> MALRGTVTDFSGFDGRADAEVLRKAMKGLGTDEDSILNLLTARSNAQRQQIAEEFKTLFGRDLVNDMKSELSGKFEKLIVALMKPSRLYDAYEL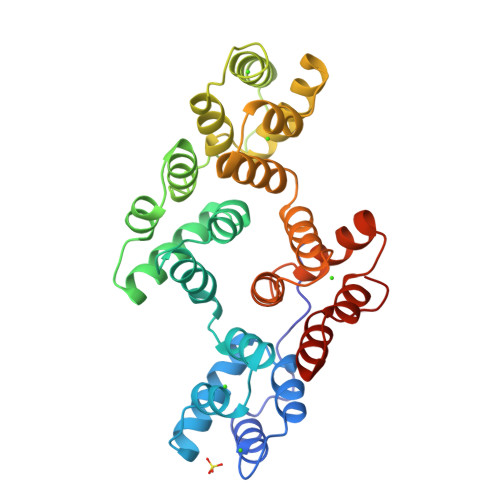KHALKGAGTDEKVLTEIIASRTPEELRAIKQAYEEEYGSNLEDDVVGDTSGYYQRMLVVLLQANRDPDTAIDDAQVELDAQALFQAGELKWGTDEEKFITILGTRSVSHLRRVFDKYMTISGFQIEETIDRETSGNLENLLLAVVKSIRSIPAYLAETLYYAMKGAGTDDHTLIRVIVSRSEIDLFNIRKEFRKNFATSLYSMIKGDTSGDYKKALLLLCGGEDD Arabidopsis thaliana (At) carboxylesterase 15 (CXE15) and carboxylesterase 20 (CXE20) have been shown to deplete strigolactones (SLs) that coordinate various growth and developmental processes and function as signaling molecules in the rhizosphere. Here, we elucidate the X-ray crystal structures of AtCXE15 (both apo and SL intermediate bound) and AtCXE20, revealing insights into the mechanisms of SL binding and catabolism. The N-terminal regions of CXE15 and CXE20 exhibit distinct secondary structures, with CXE15 characterized by an alpha helix and CXE20 by an alpha/beta fold. These structural differences play pivotal roles in regulating variable SL hydrolysis rates.

The overall architecture of AtCXE15 is divided into two domains: a cap domain (residues 1–21) and a core catalytic domain (residues 32–329), both of which are connected by a long linker loop (residues 22–31). The cap domain of CXE15 includes the NT α-helix (α1, we termed NTH) which is highly conserved among all CXE15 variants, while the catalytic domain adopts a common α/β hydrolase fold with a central nine-stranded β-sheet surrounded by ten α-helices and shares significant homology with rest of the members of CXEs. The catalytic triad consists of residues S169, H302, and E271, where the catalytic serine is positioned at the apex between α6 and β6. E271 is situated in the loop between α8 and β8 while H302 is in the loop between β9 and α10. The oxyanion hole is located above the active site within the conserved HGGGF motif, positioned in the loop between α5 and β5. Comparing the Ser-His-Asp/Glu catalytic triad sequence of all 20 CXEs revealed that in CXE15 aspartic acid is replaced by glutamic acid, making it the only CXE enzyme that is similar to the carboxylesterases in the animal kingdom. CXE15 exhibited significant hydrolytic activity compared to the catalytic mutants CXE15S169A and CXE15E271A, which were unable to hydrolyze YLG. Although CXE15ΔNTH exhibited some hydrolytic activity, its catalytic efficiency was drastically reduced to one-quarter of that of CXE15 due to the absence of the NTH. On the other hand, CXE15 exhibits a compact catalytic pocket shape, which is likely to enhance substrate specificity through specialized residues engaging with the substrate with the important contribution of NTH plasticity.

> MGSLGEEPQVAEDCMGLLQLLSNGTVLRSESIDLITQQIPFKNNQTVLFKDSIYHKPNNLHLRLYKPISASNRTALPVVVFFHGGGFCFGSRSWPHFHNFCLTLASSLNALVVSPDYRLAPEHRLPAAFEDAEAVLTWLWDQAVSDGVNHWFEDGTDVDFDRVFVVGDSSGGNIAHQLAVRFGSGSIELTPVRVRGYVLMGPFFGGEERTNSENGPSEALLSLDLLDKFWRLSLPNGATRDHHMANPFGPTSPTLESISLEPMLVIVGGSELLRDRAKEYAYKLKKMGGKRVDYIEFENKEHGFYSNYPSSEAAEQVLRIIGDFMNNLS D-MALATE 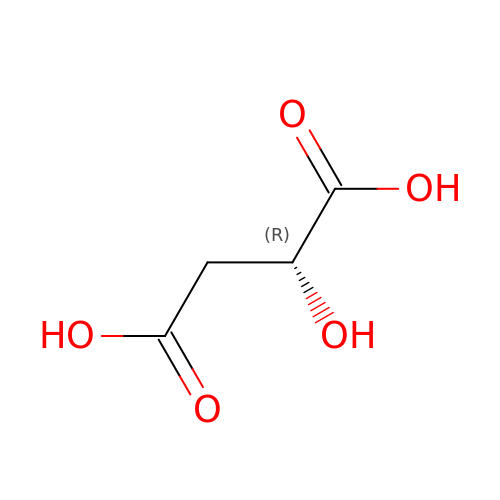| C4 H6 O5 | BJEPYKJPYRNKOW-UWTATZPHSA-N>[3x]MFEIKKICCIGAGYVGGPTCSVIAHMCPEI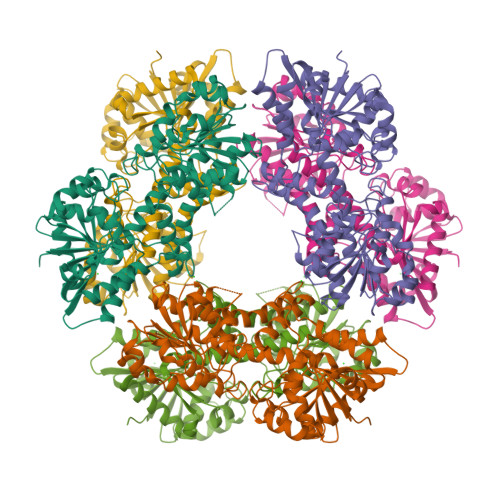RVTVVDVNESRINAWNSPTLPIYEPGLKEVVESCRGKNLFFSTNIDDAIKEADLVFISVNTPTKTYGMGKGRAADLKYIEACARRIVQNSNGYKIVTEKSTVPVRAAESIRRIFDANTKPNLNLQVLSNPEFLAEGTAIKDLKNPDRVLIGGDETPEGQRAVQALCAVYEHWVPREKILTTNTWSSELSKLAANAFLAQRISSINSISALCEATGADVEEVATAIGMDQRIGNKFLKASVGFGGSCFQKDVLNLVYLCEALNLPEVARYWQQVIDMNDYQRRRFASRIIDSLFNTVTDKKIAILGFAFKKDTGDTRESSSIYISKYLMDEGAHLHIYDPKVPREQIVVDLSHPGVSEDDQVSRLVTISKDPYEACDGAHAVVICTEWDMFKELDYERIHKKMLKPAFIFDGRRVLDGLHNELQTIGFQIETIGKKVSSKRIPYAPSGEIPKFSLQDPPNKKPKV>EIPLKYGATNEGKRQDPAMQKFRDNRLGAFIHWGLYAIPGGEWNGKVYGGAAEWLKSWAKVPADEWLKLMDQWNPTKFDAKKWAKMAKEMGTKYVKITTKHHEGFCLWPSKYTKYTVANTPYKRDILGELVKAYNDEGIDVHFYFSVMDWSNPDYRYDIKSKEDSIAFSRFLEFTDNQLKELATRYPTVKDFWFDGTWDASVKKNGWWTAHAEQMLKELVPGVAINSRLRADDKGKRHFDSNGRLMGDYESGYERRLPDPVKDLKVTQWDWEACMTIPENQWGYHKDWSLSYVKTPIEVIDRIVHAVSMGGNMVVNFGPQADGDFRPEEKAMATAIGKWMNRYGKAVYACDYAGFEKQDWGYYTRGKNDEVYMVVFNQPYSERLIVKTPKGITVEKATLLTTGEDITVVETTRNEYNVSVPKKNPGEPYVIQLKVRAAKGTKSIY[4x]

GH29 α-l-fucosidases catalyze the hydrolysis of terminal α-l-fucosidic linkages. GH29 α-l-fucosidases process their substrate with overall retention of configuration at the anomeric center of the cleaved fucopyranose and do so through a double-displacement mechanism. In this mechanism, first proposed by Koshland,, SN2 displacement of the aglycon (activated through protonation by the general acid/base residue) by nucleophilic attack of the catalytic nucleophile yields a fucosyl-enzyme intermediate, which is subsequently hydrolyzed to yield α-l-fucopyranose together with the released aglycon. Crystallographic analysis on bacterial α-l-fucosidase confirms that the ABPs act by covalent modification of the active site nucleophile.

The crystal structures of α-l-fucosidase from Bacteroides thetaiotaomicron in complex with compound 4 and 5 provide strong evidence for the covalent binding of cyclophellitol aziridine to active α-l-fucosidases and by this virtue the validity of the cyclophellitol aziridine design for activity-based profiling of retaining glycosidases that employ the Koshland double displacement mechanism. In order to minimize steric clashes, BtFuc2970 was subsequently incubated with 5. The complex has C–O bond lengths between the BtFuc2970 catalytic nucleophile and 5 of ca. 1.43 Å as would be expected for a C–O ester bond. As expected from the reduction in aglycon size, 5 is better ordered than 4 when bound to the bacterial enzyme and provides a clearer definition of the resulting conformation and interactions. Upon trans-diaxial opening of the acylaziridine the covalently bound and substituted cyclohexane adopts a slightly distorted 3H4 conformation (between 3H4 and 3S1); consistent with the expected catalytic itinerary. Whereas aziridines and epoxides that are annulated to cyclohexane rings preferably open in a trans-diaxial fashion through a chair-like transition state, reaction with the α-l-fucosidase nucleophile takes place at the aziridine carbon corresponding to the anomeric center of a substrate α-l-fucoside. This corresponds to ring opening to yield a skew boat, as is observed in the trapped enzyme active site in the co-crystal.Type IA topoisomerases (TopoIAs) are present in all living organisms. They resolve DNA/RNA catenanes, knots and supercoils by breaking and rejoining single-stranded DNA/RNA segments and allowing the passage of another nucleic acid segment through the break. Topoisomerase III-β (TOP3B), the only RNA topoisomerase in metazoans, promotes R-loop disassembly and translation of mRNAs. We present a series of cryo-EM structures of human TOP3B with its cofactor TDRD3 during cleavage and rejoining of DNA or RNA, thus elucidating the roles of divalent metal ions and key enzyme residues in each step of the catalytic cycle.

Yet, RNA complexes of TopoIA have not been previously visualized. We obtained RNA pre-cleavage and rejoining complexes of TOP3B. We anticipated that exposing cTOP3B-K10M to elevated divalent cation concentrations, known to stimulate DNA and RNA rejoining, would arrest the mutant in a rejoining conformation. Using the same strategy, we obtained a DNA post-cleavage complex with wild-type cTOP3B, and generated DNA and RNA rejoining complexes with the rejoining-deficient mutant cTOP3B-K10M10 (detailed in the corresponding section). We observed a highly similar active-site conformation for both, implying a shared mechanism of TOP3B for DNA and RNA rejoining. In addition, the presence of MnS2+ ion in both the DNA and RNA rejoining complexes underscoring its crucial role in repositioning the protein domains and nucleic acid ends for rejoining. The presence of MnS2+ in the DNA and RNA rejoining complexes suggests its essential role in aligning the cleaved DNA ends for re-ligation. Therefore, the enhanced RNA rejoining activity may relate to the ribose 2'-OH group adjacent to the nucleophile 3'-OH making it more susceptible to deprotonation.

> VMKTVLMVAEMPSLAQSIAKILSRGSLSSHKGLNGACSVHEYTGTFAGQPVRFKMTSVCGHVMTLDFLGKYNKWDKVDPAELFSQAPTEKKEANPKLNMVKFLQVEGRGCDYIVLWLDCDKEGENICFEVLDAVLPVMNKAHGGEKTVFRARFSSITDTDICNAMACLGEPDHNEALSVDARQELDLRIGCAFTRFQTKYFQGKYGDLDSSLISFGPCQTPTLGFCVERHDKIQSFKPETYWVLQAKVNTDKDRSLLLDWDRVRVFDREIAQMFLNMTKLEKEAQVEATSRKEKAKQRPLALNTVEMLRVASSSLGMGPQHAMQTAERLYTQGYISYPRTETTHYPENFDLKGSLRQQANHPYWADTVKRLLAEGINRPRKGHDAGDHPPITPMKSATEAELGGDAWRLYEYITRHFIATVSHDCKYLQSTISFRIGPELFTCSGKTVLSPGFTEVMPWQSVPLEESLPTCQRGDAFPVGEVKMLEKQTNPPDYLTEAELITLMEKHGIGTDASIPVHINNICQRNYVTVESGRRLKPTNLGIVLVHGYYKIDAELVLPTIRSAVEKQLNLIAQGKADYRQVLGHTLDVFKRKFHYFVDSIAGMDELMEVSF;> MAQVAGAALSQAGWYLSDEGIEACTSSPDKVNVNDIILIALNTDLRTIGKKFLPSDINSGKVEKLEGPCVLQIQKIRNVAAPKDNEESQAAPRMLRLQMTDGHISCTAVEFSYMSKISLNTPPGTKVKLSGIVDIKNGFLLLNDSNTTVLGGEVEHLIEKW>MSPILGYWKIKGLVQPTRLLLEYLEEKYEEHLYERDEGDKWRNKKFELGLEFPNLPYYIDGDVKLTQSMAIIRYIADKHNMLGGCPKERAEISMLEGAVLDIRYGVSRIAYSKDFETLKVDFLSKLPEMLKMFEDRLCHKTYLNGDHVTHPDFMLYDALDVVLYMDPMCLDAFPKLVCFKKRIEAIPQIDKYLKSSKYIAWPLQGWQATFGGGDHPPKSDLEVLFQGPLGSGGGGGMALVTVPTATTRLRNF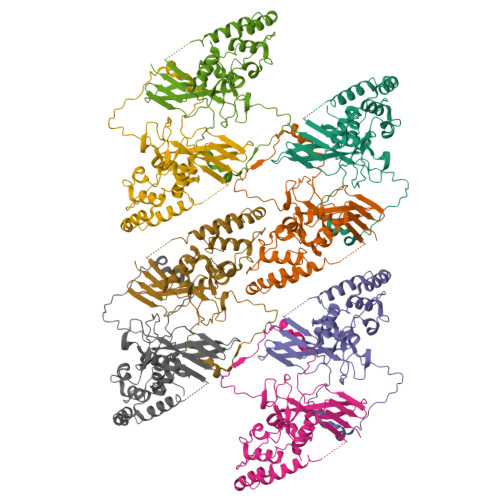CVFSSVKPLDFCDQYSSPCSSDATVDDGWFVCEYHASRFFKMEKLALAIPDGTGNNYYRTVGKSLVDDKAEGIERILIPSQNNYETVLNLSLLGPAERLVFYMIYDNKEKQNEICQQLRMYERFRPEVVEELYNSTLRVLALTNPDAYCAQTNTNESRSFGLSVEDDLAFNVLPTFIQNLIRKCVAPESLTIGTEDLQLRNANTCRITSEGLLASVRLYNSVQPKYLYGVNENRLQIRNVLQFQGNANALQQKLSRYELYQINIPLFLGKQIISTGR[8x]>MEF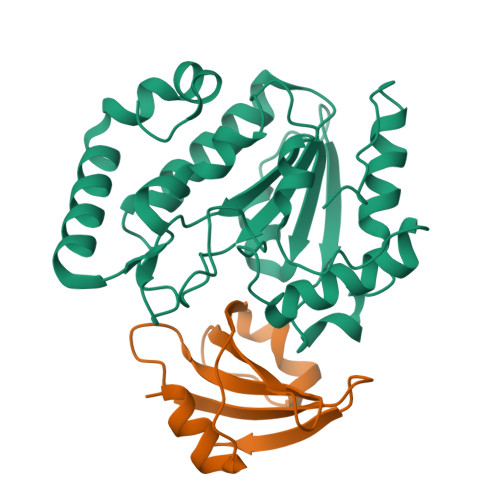FGETWRRELAAEFEKPYFKQLMSFVADERSRHTVYPPADQVYSWTEMCDIQDVKVVILGQDPYHGPNQAHGLCFSVQKPVPPPPSLVNIYKELCTDIDGFKHPGHGDLSGWAKQGVLLLNAVLTVRAHQANSHKDRGWETFTDAVIKWLSVNREGVVFLLWGSYAHKKGATIDRKRHHVLQAVHPSPLSAHRGFLGCKHFSKANGLLKLSGTEPINWRAL[8x];>MTNLSDIIEKETGKQLVIQESILMLPEEVEEVIGNKPESDILVHTAYDESTDENVMLLTSDAPEYKPWALVIQDSNGENKIKML[8x]> MRV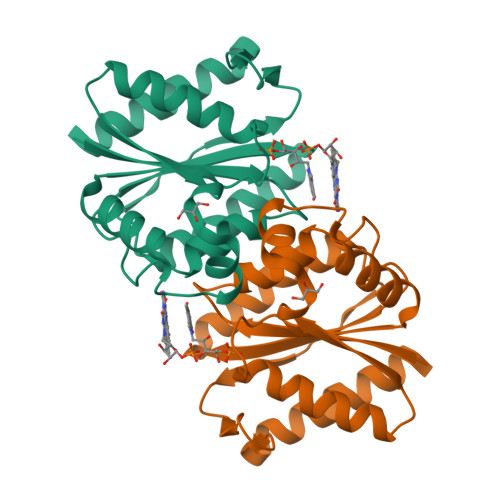ITLAGSPRFPSRSSSLLEYAREKLNGLDVEVYHWNLQNFAPEDLLYARFDSPALKTFTEQLQQADGLIVATPVYKAAYSGALKTLLDLLPERALQGKVVLPLATGGTVAHLLAVDAALKPVLSALKAQEILHGVFADDSQVIDYHHRPQFTPNLQTRLDTALETFWQALHRRDVQVPDLLSLRGNAHA>[2x]AHMFMAENRLQ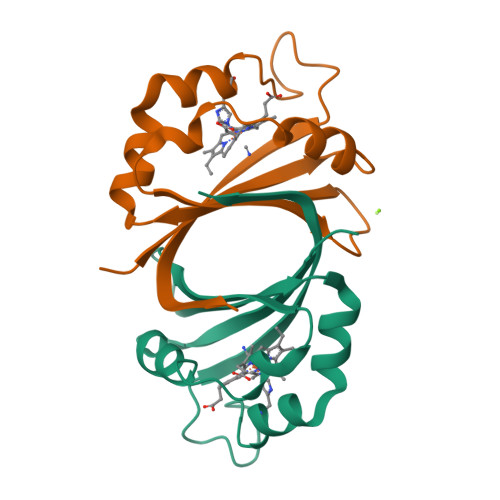LQKGSAEETIERFYNRQGIETIEGFQQMFVTKTLNTEDTDEVKILTIWESEDSFNNWLNSDVFKEAHKNVRLKSDDDGQQSPILSNKVFKYDIGYHYQK> MDEIDLRILKILQYNAKYSLDEIAREIRIPKSTLSYRIKKLEKDGVIKGYYAYINPASLNLDYIVITSVKAKYGKNAHVELG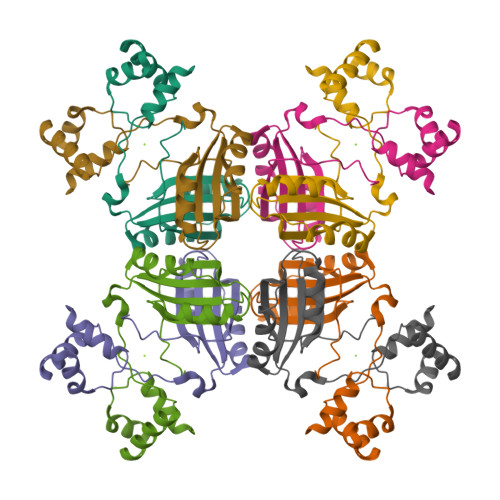NKLAQIPGVWGVYFVLGDNDFIVMARYKTREEFMEKFLERVMSIPEVERTSTQVVVKIIKESPNIVIF~{N}-[3-[(dimethylamino)methyl]-5-methyl-phenyl]-2-[3-methoxy-5-(7-methoxyquinolin-4-yl)oxy-pyridin-2-yl]ethanamide | C28 H30 N4 O4 | 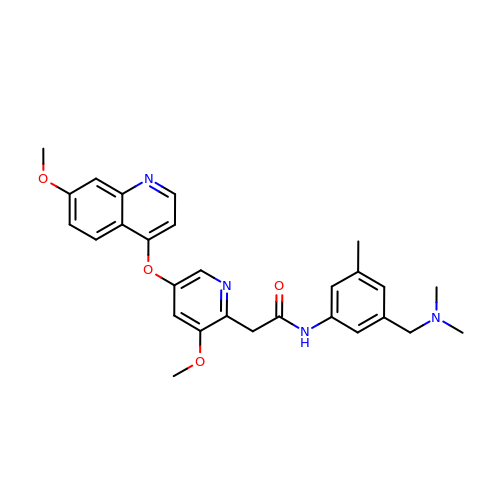MALCRTBNJLPDJJ-UHFFFAOYSA-N>[4x]QVIEVLNKQVADWSVLFTKLHNFHWYVKGPQFFTLHEKFEELYTESA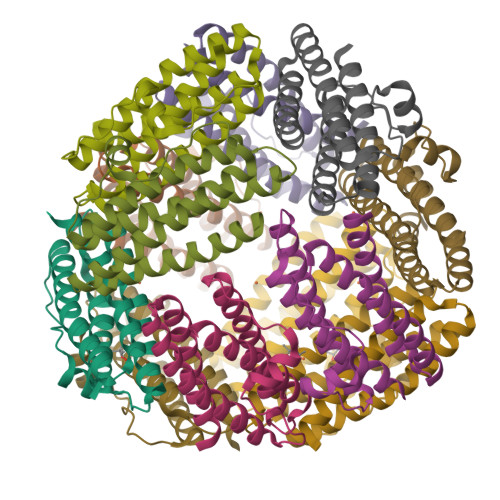THIDEIAERILAIGGKPVATMKEYLEISSIQEAAYGETAEGMVEAIMKDYEMMLVELKKGMEIAQNSDDEMTSDLLLGIYTELEKHAWMLRAFLN>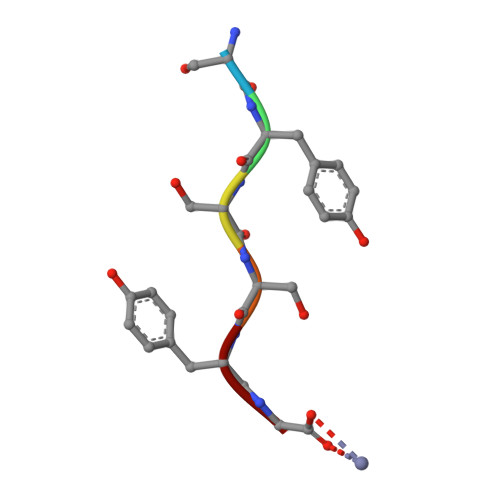 SYSSYG>[2x]GPMPKRLINKNIDIYNYPNEFEDNLGSISLGDLHGNAIKLIHFLFRHKIIKFKTEIINFHEAYQQFVTIYEQYDDMVQEYLEIRTLLQLIQIKITNAQQRILDIEQKLSLATDHQKEFSQSLLQLKKPIEANLQMAEKSKAGLEEKLSGLKTRLPSCIERFNKFMTQIEINDIKTLIRLLGDEVADRGSCDYFTLRIL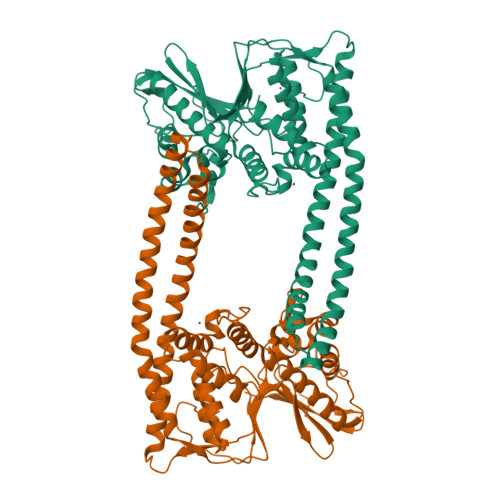DFLYQNQIAIKIILSNHGYEFIHAYEKLVVGQPFKPKGYIGDIQIKSFWGLQLLLEQSVITEEELRSLVERAYKPTLKIIDYSLSEDGITLYSHAPIRFDSIRMAASQLGVTYNDSTKEALAETIDQLNAQLQIYMKNNMLHLLFENNEINDPTNMTDEERNASPLIYLVWNRWNESKEVENARPGKYNGYFVTYVHGHDPFQSPLTYVYNLDT> GAEFMDLDQGGEALAPRQVLDLEDLVFTQGSHFMANKRCQLPDGSFRRQRKGYEEVHVPALKPKPFGSEEQLLPVEKLPKYAQAGFEGFKTLNRIQSKLYRAALETDENLLLCAPTGAGKTNVALMCMLREIGKHINMDGTINVDDFKIIYIAPMRSLVQEMVGSFGKRLATYGITVAELTGDHQLCKEEISATQIIVCTPEKWDIITRKGGERTYTQLVRLIILDEIHLLHDDRGPVLEALVARAIRNIEMTQEDVRLIGLSATLPNYEDVATFLRVDPAKGLFYFDNSFRPVPLEQTYVGITEKKAIKRFQIMNEIVYEKIMEHAGKNQVLVFVHSRKETGKTARAIRDMCLEKDTLGLFLREGSASTEVLRTEAEQCKNLELKDLLPYGFAIHHAGMTRVDRTLVEDLFADKHIQVLVSTATLAWGVNLPAHTVIIKGTQVYSPEKGRWTELGALDILQMLGRAGRPQYDTKGEGILITSHGELQYYLSLLNQQLPIESQMVSKLPDMLNAEIVLGNVQNAKDAVNWLGYAYLYIRMLRSPTLYGISHDDLKGDPLLDQRRLDLVHTAALMLDKNNLVKYDKKTGNFQVTELGRIASHYYITNDTVQTYNQLLKPTLSEIELFRVFSLSSEFKNITVREEEKLELQKLLERVPIPVKESIEEPSAKINVLLQAFISQLKLEGFALMADMVYVTQSAGRLMRAIFEIVLNRGWAQLTDKTLNLCKMIDKRMWQSMCPLRQFRKLPEEVVKKIEKKNFPFERLYDLNHNEIGELIRMPKMGKTIHKYVHLFPKLELSVHLQPITRSTLKVELTITPDFQWDEKVHGSSEAFWILVEDVDSEVILHHEYFLLKAKYAQDEHLITFFVPVFEPLPPQYFIRVVSDRWLSCETQLPVSFRHLILPEKYPPPTELLDLQPLPVSALRNSAFESLYQDKFPFFNPIQTQVFNTVYNSDDNVFVGAPTGSGKTICAEFAILRMLLQSSEGRCVYITPMEALAEQVYMDWYEKFQDRLNKKVVLLTGETSTDLKLLGKGNIIISTPEKWDILSRRWKQRKNVQNINLFVVDEVHLIGGENGPVLEVICSRMRYISSQIERPIRIVALSSSLSNAKDVAHWLGCSATSTFNFHPNVRPVPLELHIQGFNISHTQTRLLSMAKPVYHAITKHSPKKPVIVFVPSRKQTRLTAIDILTTCAADIQRQRFLHCTEKDLIPYLEKLSDSTLKETLLNGVGYLHEGLSPMERRLVEQLFSSGAIQVVVASRSLCWGMNVAAHLVIIMDTQYYNGKIHAYVDYPIYDVLQMVGHANRPLQDDEGRCVIMCQGSKKDFFKKFLYEPLPVESHLDHCMHDHFNAEIVTKTIENKQDAVDYLTWTFLYRRMTQNPNYYNLQGISHRHLSDHLSELVEQTLSDLEQSKCISIEDEMDVAPLNLGMIAAYYYINYTTIELFSMSLNAKTKVRGLIEIISNAAEYENIPIRHHEDNLLRQLAQKVPHKLNNPKFNDPHVKTNLLLQAHLSRMQLSAELQSDTEEILSKAIRLIQACVDVLSSNGWLSPALAAMELAQMVTQAMWSKDSYLKQLPHFTSEHIKRCTDKGVESVFDIMEMEDEERNALLQLTDSQIADVARFCNRYPNIELSYEVVDKDSIRSGGPVVVLVQLEREEEVTGPVIAPLFPQKREEGWWVVIGDAKSNSLISIKRLTLQQKAKVKLDFVAPATGAHNYTLYFMSDAYMGCDQEYKFSVDVKEAETDSDSD

BRR2 is responsible for the unwinding of U4/U6 di-small nuclear (sn) RNAs, an essential step for the conversion of a pre-catalytic spliceosome (B complex) to an activated spliceo­some (Bact complex; Raghunathan & Guthrie, 1998; Laggerbauer et al., 1998). The ∼250 kDa enzyme is composed of an N-terminal auto-regulatory region of about 400 residues and tandem helicase cassettes, each comprising two RecA-like domains (RecA1 and RecA2), a winged-helix (WH) domain, a helical bundle (HB) or ratchet domain, a helix–loop–helix (HLH) domain and an immunoglobulin-like (IG) domain. Due to its essential role in each splicing event and its association with the genetically inherited visual deficiency retinitis pigmentosa, BRR2 is an interesting target for the development of small-molecule modulators.

We identified sulfaguanidine [4-amino-N-(aminoiminomethyl)-benzolsulfonamide], a known antibacterial drug, as a ligand of hBRR2T1 in a crystallization screen with additives (Silver Bullets condition 12; Hampton Research, catalogue No. HR2-096). In this hBRR2T1 crystal structure, sulfaguanidine is positioned at the interface between the two helicase cassettes, directly contacting the N-terminal HB and IG domains as well as the C-terminal RecA2 domain. The para-positioned amino group forms a hydrogen bond to Glu1097 of the HB domain and the guanidine moiety is contacted by a hydrogen bond to the main chain of His1236 of the IG domain. Furthermore, the binding is supported by π-stacking interactions with Tyr1238 and van der Waals interactions of the benzene ring with Trp1222 (N-terminal IG domain) and Asn1531 (N-terminal RecA2 domain). Sulfaguanidine occupies a different binding site displaced by about 9 Å from BRR2-inhibitory compounds and did not influence the RNA helicase activity of hBRR2T1. The primary hot spot (16 interacting probes) is located at the interface between the cassettes, coinciding with the position of known hBRR2 inhibitors. A second hot spot (13 interacting probes) overlaps with the original sulfaguanidine-binding site. While compound 33a efficiently inhibited hBRR2T1-mediated U4/U6 unwinding (45% of the unwinding amplitude of the DMSO control after 2 min), we did not detect any effect of sulfaguanidine on unwinding at 300 µM or 1 mM. Sulfaguanidine itself did not bind to the hBRR2T1–hJab1ΔC crystals.>[2x]MASEDKNIIHGPPPFYSLDIGTAGEQLHKFMKKYAQITGTIAFTDAHNGVNVTYAEYFEMACRLAQSMKNYGLTLKHRIAVCSENSLQFFMPICGALFIGVGVAPTNDIYNERELYNSLGISQPTIVFCSKRALQKILGVQQKLPIIEKIIILDSQEDFMGKQSMNSFIRQFLPETFNEYDYVPDSFALNTTAFIMNSSGSTGLPKGVDLTHQNIVVRFSHCRDPIFGNQIIPDTSILSVIPFHHGFGMSTTLGYLVCGFRIVLMYRFEEELFLRSLQNYKCQSALLVPTLFSFFAKSTLVDKYDLSNLHEVASGGAPLAKEVGEAVAKRFNLVGIRQGYGLTETTSACIITPEGDNKPGACGKVVPFFSAKVTDLDTGKTLGPNQRGELWLKGPMVMKGYVNNPEATHSLI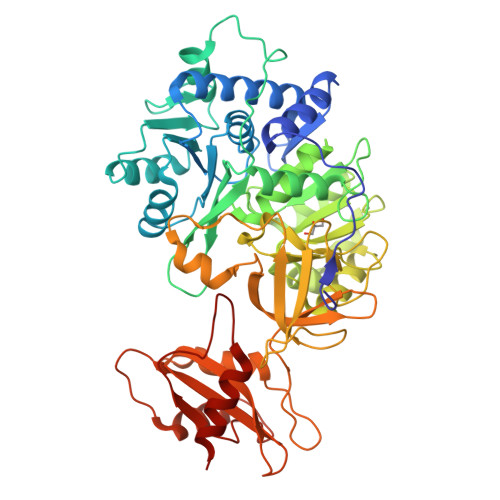DKEGWVRTGDIAYYDEDEHFFIVDRLKSLIKYKGYQVPPAELESILLQHPYIFDAGVAGIPDPDAGELPAAVVVLEEGKTMTEKEVMDYVAGQVTSSKRLRGGVKFVDEVPKGLTGKIDGRKIREILLKAKKSKL[(ISOQUINOLIN-1-YLAMINO)-PHOSPHONO-METHYL]-PHOSPHONIC 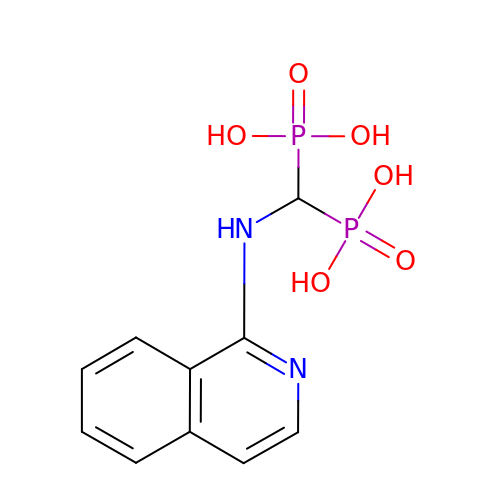ACID | C10 H12 N2 O6 P2 | JPVMIOWESIQIGB-UHFFFAOYSA-N>MLVKGNEILLKAHKEGYGVGAFNFVNFEMLNAIFEAGNEENSPLFIQASEGAIKYMGIDMAVGMVKIMCERYPHIPVALHLDHGTTFESCEKAVKAG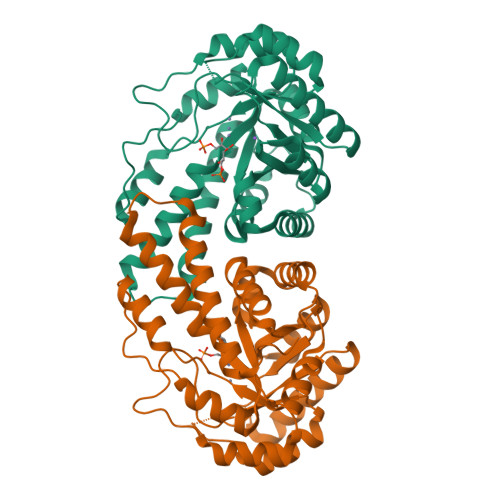FTSVMIDASHHAFEENLELTSKVVKMAHNAGVSVEAELGRLMGIADNISVDEKDAVLVNPKEAEQFVKESQVDYLAPAIGTSHGAFKFKGEPKLDFERLQEVKRLTNIPLVLHGASAIPDNVRKSYLDAGGDLKGSKGVPFEFLQESVKGGINKVNTDTDLRIAFIAEVRKVANEDKSQFDLRKFFSPAQLALKNVVKERMKLLGSANKI[2x]> GPQRTCGSELNMEQIRRTEPLKYQRITDWENQIKLHSRSVPSSTIL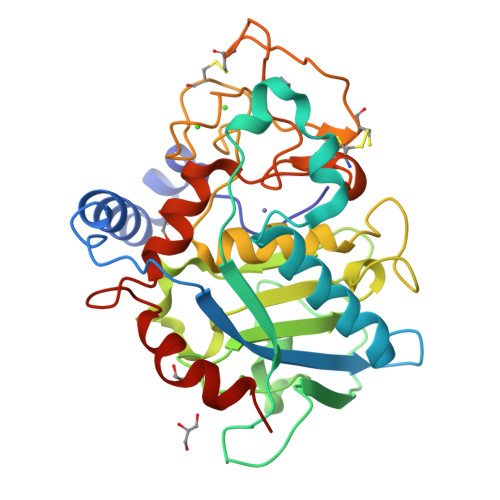IPVVVHVVYNNSAQNISDAQIISQIQVLNEDFRRMNADQANTPSAFANLAGNANIEFKLARRDPNGNTTNGITRTSTSTETFSMEMDNVKFSNLGGNNAWNTRRYLNIWVCNLGDDLLGYAQFPFEFQTKPNTDGVVIHYKHFGRDGSAESPYDKGRTATHAVGHWLDLRHIWGDDGGSCSGTDNIADTPNQGGYNEGCPSFPKTDHCTNTSPGVMFMNYMDYTYDACMNLFTKGQVERMRSLFDTQTGIRREMQIYANELTNPLSFS> MTKKVGLLVMAYGTPYKDEDIERYYTDIRHGHKPSEEMIADLRGLYHAIGGLSPLAKITEAQAYGLEKALNDSQDEVEFKAYIGLKHIEPFIEDAVEAMHKDGIEEAISIVLAPHYSSFSVEAYNKRAKEAADKLGGPRINAINDWYKQPKFIQMWADRINETAKQIPADELLDTVLIVSAHSLPEKIKQHNDPYPNQLQETADFIFEKVVVPHYALGWQSEGKTGEPWLGPDVQDLTRELYGREKYKHFIYTPVGFVAEHLEVLYDNDYECKVVTDEVGAAYHRPPMPNSDPEFLEVLRTVVWEKYSNLE

Coproporphyrin ferrochelatases (CpfCs) are enzymes catalyzing the penultimate step in the coproporphyrin‐dependent (CPD) heme biosynthesis pathway, which is mainly utilized by monoderm bacteria. Here Fe2+ ion is incorporated into coproporphyrin III (cpIII) to give Fe3+‐coproheme, which is afterwards decarboxylated by the coproheme decarboxylase enzyme, finally yielding protoheme. A cleft, build by structural elements of both ferredoxin‐like domains, contains several conserved amino acid residues (distal H182 and E263; proximal Y12) and is the porphyrin binding site, where catalysis happens, as already shown for CpfC from Bacillus subtilis. Here, we present the first crystallographic structure of the CpfC from the representative monoderm pathogen Listeria monocytogenes bound to its physiological substrate, cpIII, together with the in‐solution data obtained by resonance Raman and UV–vis spectroscopy, for wild‐type ferrochelatase and variants, analyzing propionate interactions.

The structures of LmCpfC wild‐type (WT) and of the R45L variant were solved in complex with the natural substrate cpIII. The R45L variant was investigated since, lacking the H‐bonding with the propionate at position 6 (p6), highlights the importance of this propionate interaction in LmCpfC. Diffraction data for LmCpfC wild‐type and for the R45L variant were collected to 1.51 Å and 2.64 Å resolution, respectively. 11 When bound to the enzyme, cpIII is distorted leading to a distinctly non‐planar geometry in both the wild‐type protein and the R45L variant. Some uncertainty remains on the detailed orientation of the carboxyl groups of the more flexible propionate p6 and p7 in the structure of cpIII‐LmCpfC R45L, due to weak electron densities. Nevertheless, the spatial orientation of the propionates towards the respective H‐bonding partners can be identified also in the R45L variant. The cpIII‐R45L (LmCpfC) crystal structure shows that, in the absence of the R45‐p6 H‐bond, the R29‐p7 H‐bond length changes from 2.9 Å in the WT to 5.9 Å in the R45L mutant. The similarity between the spectra of R29L and R45L can be rationalized considering the concomitant destabilizing effect on the R29‐p7 interaction by the R45L mutation, where the H‐bond with p6 has been eliminated. In solution the loss of the p6‐R45 H‐bond causes a dramatic weakening of the whole H‐bond network, since in addition to the rupture of the H‐bond between p7 and R29, it also makes the H‐bond between p2 and Y124 much weaker, as compared to the WT (downshift of the 403 cm−1 mode in the WT to 393 cm−1 in the mutant). The crystallographic data suggest that p6 and p7 are coupled, and the RR in solution clearly indicate that an overall readjustment of the propionate H‐bonds occurs as well in both R45L and R29L variants.> MASDNLSAVLYKQNDLRLEQRPIPEPKEDEVLLQMAYVGICGSDVHYYEHGRIADFIVKDPMVIGHEASGTVVKVGKNVKHLKKGDRVAVEPGVPCRRCQFCKEGKYNLCPDLTFCATPPDDGNLARYYVHAADFCHKLPDNVSLEEGALLEPLSVGVHACRRAGVQLGTTVLVIGAGPIGLVSVLAAKAYGAFVVCTARSPRRLEVAKNCGADVTLVVDPAKEEESSIIERIRSAIGDLPNVTIDCSGNEKCITIGINITRTGGTLMLVGMGSQMVTVPLVNACAREIDIKSVFRYCNDYPIALEMVASGRCNVKQLVTHSFKLEQTVDA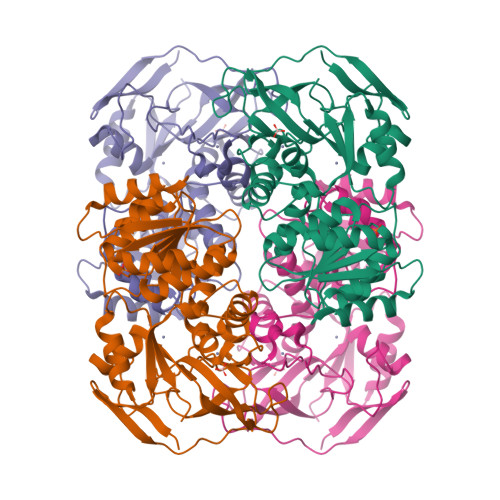FEAARKKADNTIKVMISCRQG3-methyl-1-(oxan-4-yl)-8-pyridin-3-yl-imidazo[4,5-c]quinolin-2-one | C21 H20 N4 O2 | 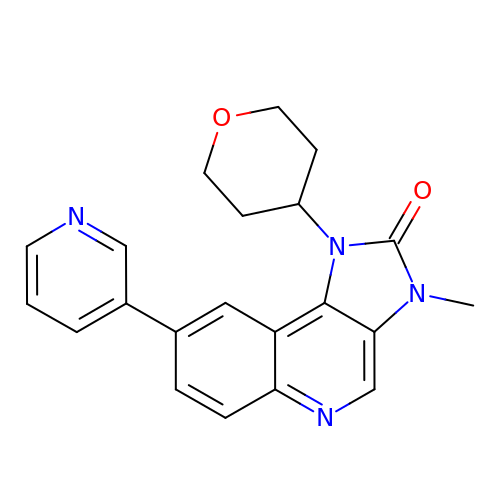QPTLAOOZWOLYLB-UHFFFAOYSA-N> GKITLYEDRGFQGRHYECSSDHPNLQPYLSRCNSARVDSGCWMLYEQPNYSGLQYFLRRGDYADHQQWMGLSDSVRSCRLIPHSGSHRIRLYEREDYRG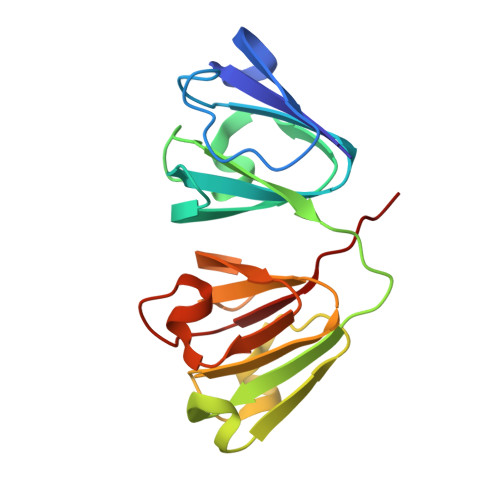QMIEFTEDCSMLQDRFRFNEIHSLNVLEGSWVLYELSNYRGRQYLLMPGDYRRYQDWGATNARVGSLRRVIDFS2-amino-5-[(Z)-iminomethyl]-3,7-dihydro-4H-pyrrolo[2,3-d]pyrimidin-4-one | C7 H7 N5 O | 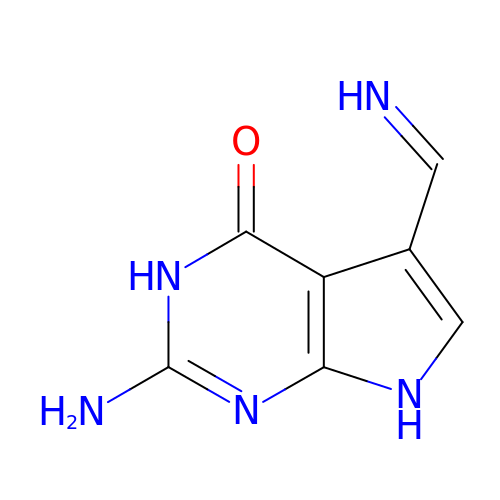BETPBINTBSWYLZ-QPIMQUGISA-N> GPHMASKSEQLLIVVSILEGRQFPRSPRLSLVVEARFDGETLSTDPVEHKEQPQFCTELAWELDRRTLHQHRLQRTPIKLQCYAVDSSTSARESVGYIVLDLRSVQEIKQAPKWHPLLSSKYTKLKPALLIGMILENDN

Using X-ray crystallography, we show that the ciliopathy-associated centriolar protein CEP120 contains three C2 domains. CEP120, for example, plays a key role in the duplication, elongation, and maturation of centrioles, which in principle could impact the production of a functional basal body (Comartin et al., 2013, Lin et al., 2013, Mahjoub et al., 2010, Wu et al., 2014). All three C2 domains of CEP120 (C2A, C2B, and C2C) adopt the PLC δ1-like topology II and are structurally similar to each other (root-mean-square deviation [RMSD], 2.4–2.6 Å), with major differences found mainly in their loop length. Thus, the CEP120 C2 domains probably play a role as protein-protein interaction modules.

While the C2A domain of CEP120 interacts with tubulin and promotes microtubule formation (Lin et al., 2013, Sharma et al., 2018), our results suggest that the C2B domain does not directly contribute to this activity, as neither JS nor JATD mutations in C2B abolished the ability of CEP120 to cause centriole overextension when overexpressed in cells. Our structures revealed neither complexed Ca2+ nor potential Ca2+-coordinating top loop residues or cationic β-grooves.Survival of motor neuron (SMN) functions in diverse biological pathways via recognition of symmetric dimethylarginine (Rme2s) on proteins by its Tudor domain, and deficiency of SMN leads to spinal muscular atrophy. Here we report a potent and selective antagonist with a 4-iminopyridine scaffold targeting the Tudor domain of SMN. In order to understand the structural basis of compound 1 recognition by these reader proteins, we determined the crystal structures of compound 1 in complex with SMN, TDRD3 and UHRF1, respectively. In this study, we identified some low micromolar antagonists with a 4-iminopyridine scaffold targeting the Tudor domain of SMN, and compound 1 shows >4-fold selectivity over other tested methyllysine or methylarginine binding domains.

In the complex structure of SMN-compound 1, compound 1 binds to the aromatic cage formed by W102, Y109, Y127 and Y130, which otherwise accommodates dimethylarginine of its physiological ligands. W102 and Y130 sandwich compound 1 rings. In addition, compound 1 forms a hydrogen bond between its imino group and the side chain of N132. This hydrogen bond boosts the ligand binding ability of SMN, because mutating N132 to alanine significantly reduced its binding affinity. In addition, the W102A and Y130A mutants of SMN did not bind to compound 1. On the other hand, the mutations of the SMN cage residues Y109 and Y127 weakened, but did not abrogate the binding of SMN to compound 1. Hence, the sandwich stacking interactions of compound 1 by W102 and Y130 of SMN play a more critical role in the specific compound 1 recognition by SMN. Due to the electronic similarity between the N-methyl and 4-imino sites on the 4-iminopyridine core, we did not expect to resolve the orientation of compound 1 based on electron density alone, and could not exclude the possibility that the imino group would instead protrude into the solvent. However, the positive binding results of 1-substituted pyridine cores to SMN presented here could confirm that N132 does interact with the imino group and substituents on the pyridine nitrogen would point away from the Tudor domain, as larger 1-substituents would otherwise clash inside the aromatic cage. Although the binding affinity of SMN and compound 1 is not high, SMN binds to compound 1 60–180-fold more tightly than its physiological ligands such as symmetric dimethylarginine or R1810me2s-POLR2A (Kd of 2.6 μM for compound 1 vs 476 μM for symmetric dimethylarginine or 175 μM for R1810me2s-POLR2A9).

> GKKNTAASLQQWKVGDKCSAIWSEDGCIYPATIASIDFKRETCVVVYTGYGNREEQNLSDLLSPICE> MTTYSDKGAKPERGRFLHFHSVTFWVGNAKQAASFYCSKMGFEPLAYRGLETGSREVVSHVIKQGKIVFVLSSALNPWNKEMGDHLVKHGDGVKDIAFEVEDCDYIVQKARERGAKIMREPWVEQDKFGKVKFAVLQTYGDTTHTLVEKMNYIGQFLPGYEAPAFMDPL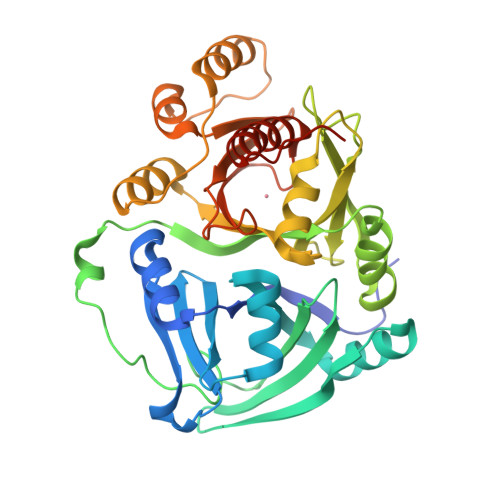LPKLPKCSLEMIDHIVGNQPDQEMVSASEWYLKNLQFHRFWSVDDTQVHTEYSSLRSIVVANYEESIKMPINEPAPGKKKSQIQEYVDYNGGAGVQHIALKTEDIITAIRHLRERGLEFLSVPSTYYKQLREKLKTAKIKVKENIDALEELKILVDYDEKGYLLQIFTKPVQDRPTLFLEVIQRHNHQGFGAGNFNSLFKAFEEEQNLRGNLTNMETNGVVPGM>[6x]GTKQEKTILNMARFIRSQALTILEKANELDADEIADIAESIHDHADEIYRSALARFGD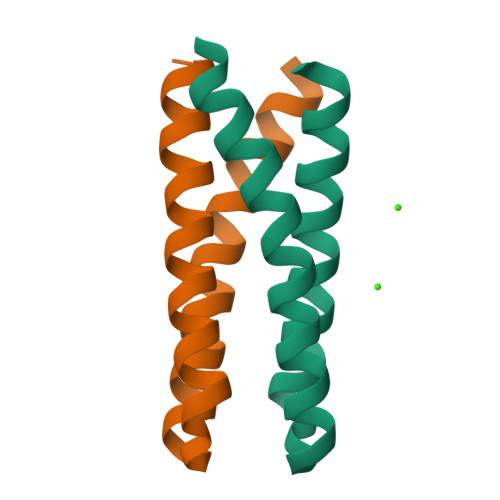DGENL> MEVHDFETDEFNDFNEDDYATREFLNPDERMTYLNHADYNLNSPLISDDIDNLIRKFNSLPIPSMWDSKNWDGVLEMLTSCQANPISTSQMHKWMGSWLMSDNHDASQGYSFLHEVDKEAEITFDVVETFIRGWGNKPIEYIKKERWTDSFKILAYLCQKFLDLHKLTLILNAVSEVELLNLARTFKGKVRRSSHGTNICRIRVPSLGPTFISEGWAYFKKLDILMDRNFLLMVKDVIIGRMQTVLSMVCRIDNLFSEQDIFSLLNIYRIGDKIVERQGNFSYDLIKMVEPICNLKLMKLARESRPLVPQFPHFENHIKTSVDEGAKIDRGIRFLHDQIMSVKTVDLTLVIYGSFRHWGHPFIDYYTGLEKLHSQVTMKKDIDVSYAKALASDLARIVLFQQFNDHKKWFVNGDLLPHDHPFKSHVKENTWPTAAQVQDFGDKWHELPLIKCFEIPDLLDPSIIYSDKSHSMNRSEVLKHVRMNPNTPIPSKKVLQTMLDTKATNWKEFLKEIDEKGLDDDDLIIGLKGKERELKLAGRFFSLMSWKLREYFVITEYLIKTHFVPMFKGLTMADDLTAVIKKMLDSSSGQGLKSYEAICIANHIDYEKWNNHQRKLSNGPVFRVMGQFLGYPSLIERTHEFFEKSLIYYNGRPDLMRVHNNTLINSTSQRVCWQGQEGGLEGLRQKGWTILNLLVIQREAKIRNTAVKVLAQGDNQVICTQYKTKKSRNVVELQGALNQMVSNNEKIMTAIKIGTGKLGLLINDDETMQSADYLNYGKIPIFRGVIRGLETKRWSRVTCVTNDQIPTCANIMSSVSTNALTVAHFAENPINAMIQYNYFGTFARLLLMMHDPALRQSLYEVQDKIPGLHSSTFKYAMLYLDPSIGGVSGMSLSRFLIRAFPDPVTESLSFWRFIHVHARSEHLKEMSAVFGNPEIAKFRITHIDKLVEDPTSLNIAMGMSPANLLKTEVKKCLIESRQTIRNQVIKDATIYLYHEEDRLRSFLWSINPLFPRFLSEFKSGTFLGVADGLISLFQNSRTIRNSFKKKYHRELDDLIVRSEVSSLTHLGKLHLRRGSCKMWTCSATHADTLRYKSWGRTVIGTTVPHPLEMLGPQHRKETPCAPCNTSGFNYVSVHCPDGIHDVFSSRGPLPAYLGSKTSESTSILQPWERESKVPLIKRATRLRDAISWFVEPDSKLAMTILSNIHSLTGEEWTKRQHGFKRTGSALHRFSTSRMSHGGFASQSTAALTRLMATTDTMRDLGDQNFDFLFQATLLYAQITTTVARDGWITSCTDHYHIACKSCLRPIEEITLDSSMDYTPPDVSHVLKTWRNGEGSWGQEIKQIYPLEGNWKNLAPAEQSYQVGRCIGFLYGDLAYRKSTHAEDSSLFPLSIQGRIRGRGFLKGLLDGLMRASCCQVIHRRSLAHLKRPANAVYGGLIYLIDKLSVSPPFLSLTRSGPIRDELETIPHKIPTSYPTSNRDMGVIVRNYFKYQCRLIEKGKYRSHYSQLWLFSDVLSIDFIGPFSISTTLLQILYKPFLSGKDKNELRELANLSSLLRSGEGWEDIHVKFFTKDILLCPEEIRHACKFGIAKDNNKDMSYPPWGRESRGTITTIPVYYTTTPYPKMLEMPPRIQNPLLSGIRLGQLPTGAHYKIRSILHGMGIHYRDFLSCGDGSGGMTAALLRENVHSRGIFNSLLELSGSVMRGASPEPPSALETLGGDKSRCVNGETCWEYPSDLCDPRTWDYFLRLKAGLGLQIDLIVMDMEVRDSSTSLKIETNVRNYVHRILDEQGVLIYKTYGTYICESEKNAVTILGPMFKTVDLVQTEFSS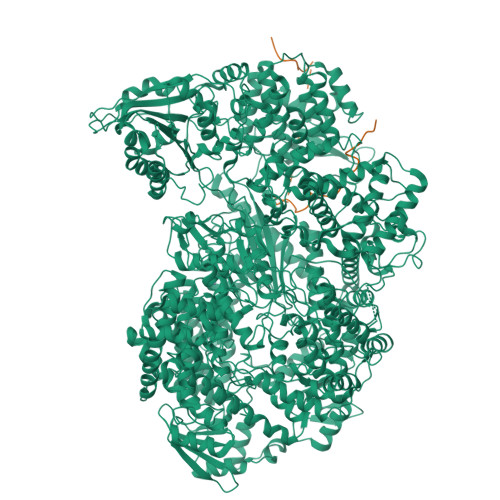SQTSEVYMVCKGLKKLIDEPNPDWSSINESWKNLYAFQSSEQEFARAKKVSTYFTLTGIPSQFIPDPFVNIETMLQIFGVPTGVSHAAALKSSDRPADLLTISLFYMAIISYYNINHIRVGPIPPNPPSDGIAQNVGIAITGISFWLSLMEKDIPLYQQCLAVIQQSFPIRWEAVSVKGGYKQKWSTRGDGLPKDTRISDSLAPIGNWIRSLELVRNQVRLNPFNEILFNQLCRTVDNHLKWSNLRRNTGMIEWINRRISKEDRSILMLKSDLHEENSWRD;> MDNLTKVREYLKSYSRLDQAVGEIDEIEAQRAEKSNYELFQEDGVEEHTKPSYFQAADDSDTESEPEIEDNQGLYAQDPEAEQVEGFIQGPLDDYADEEVDVVFTSDWKPPELESDEHGKTLRLTSPEGLSGEQKSQWLSTIKAVVQSAKYWNLAECTFEASGEGVIMKERQITPDVYKVTPVMNTHPSQSEAVSDVWSLSKTSMTFQPKKASLQPLTISLDELFSSRGEFISVGGDGRMSHKEAILLGLRYKKLYNQARVKYSL>AQVINTFDGVADYLQTYHKLPDNYITKSEAQALGWVASKGNLADVAPGKSVGGDIFSNREGKLPGKSGRTWREADINYTSGFRNSDRILYSSDWLIYKTTDHYQTFTKIR[3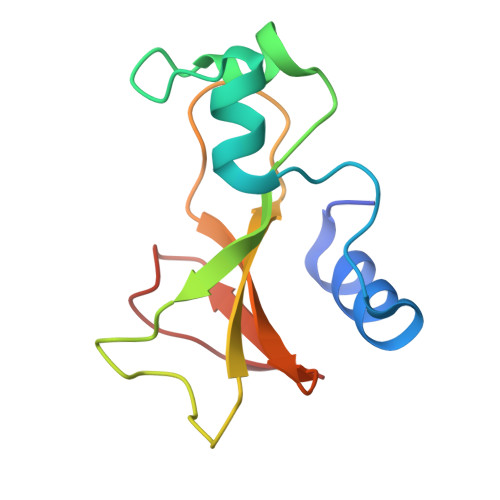x]> MSRLMPHYSKGKTAFLCVDLQEAFSKRIENFANCVFVANRLARLHELVPENTKYIVTEHYPKGLGRIVPGITLPQTAHLIEKTRFSCIVPQVEELLEDVDNAVVFGIEGHACILQTVADLLDMNKRVFLPKDGLGSQKKTDFKAAMKLMGSWSPNCEITTSESILLQMTKDAMDPNFKKISKLLKEEPP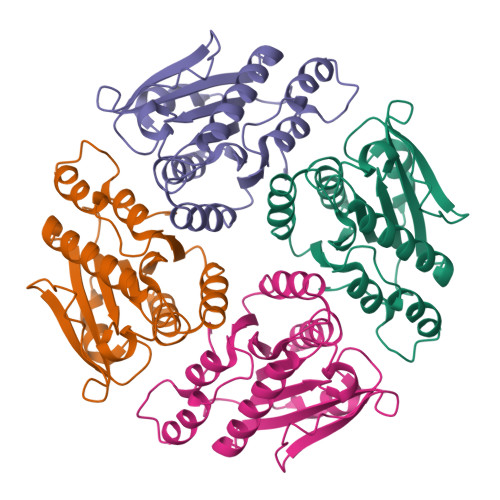IPL> MKHHHHHHPMATDLGSFKANFIDSDGNQMTDVVEINFADATEKNISNLLNTLLGRDREEFTPYRFRIHIPGKDLIIDQYPNDLL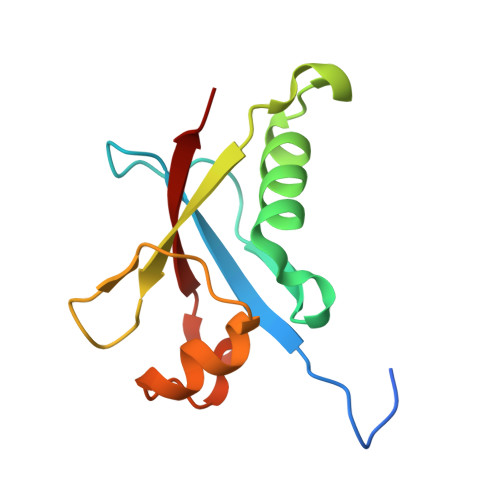SLLQKHGVTNPFETTITLSAEPQA>MRSDAMSGQMFKVEIVTRPANFEKLKQELGKIGVTSLTFSNVHGCGLQKAHTELYRGVKIESNVYERLKIEIVVSKVPVDQVTETAKRVLKTGSPGDGKIFVYEISNTINIRTGEEGPEAL[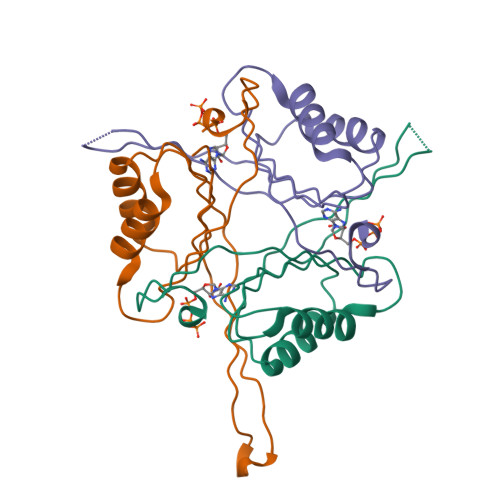3x]> MKMFFRLTRELRDELKRPLGELVRGPIPEPYLKVRGELEKHPVVTVGDVVTENVLKIGVKPIIALYDLKTKRKEYSPEIEDTAVFLTVTNPPGTITKALLDTVRKAFGLAERGRNVHILVSGEEDLAAIPAVLYAPLGTLVLYGQP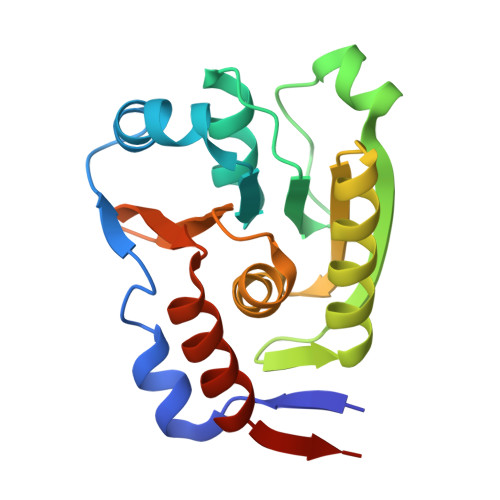DEGVVLIKVTPECKRRCAKILASMEVVRDGD> DSLRPKLSEEQQRIIAILLDAHHKTYDPTYSDFCQFRPPVRVNDGGGSVTLELSQLSMLPHLADLVSYSIQKVIGFAKMIPGFRDLTSEDQIVLLKSSAIEVIMLRSNESFTMDDMSWTCGNQDYKYRVSDVTKAGHSLELIEPLIKFQVGLKKLNLHEEEHVLLMAICIVSPDRPGVQDAALIEAIQDRLSNTLQTYIRCRHPPPGSHLLYAKMIQ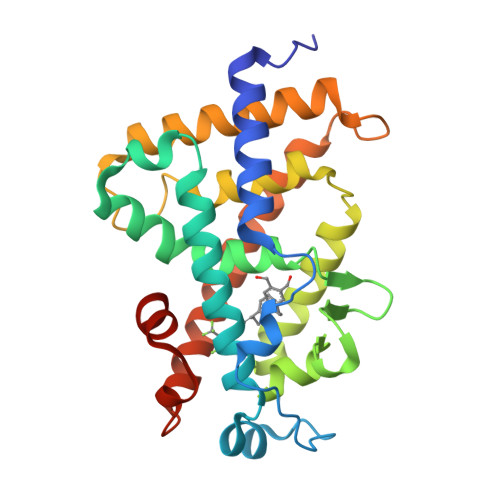KLADLRSLNEEHSKQYRCLSFQPECSMKLTPLVLEVFGNEIS> MGFLPQAQGGGAAASAKVSGTRFVIDGKTGYFAGTNSYWIGFLTNNRDVDTTLDHIASSGLKILRVWGFNDVNNQPSGNTVWFQRLASSGSQINTGPNGLQRLDYLVRSAETRGIKLIIALVNYWDDFGGMKAYVNAFGGTKESWYTNARAQEQYKRYIQAVVSR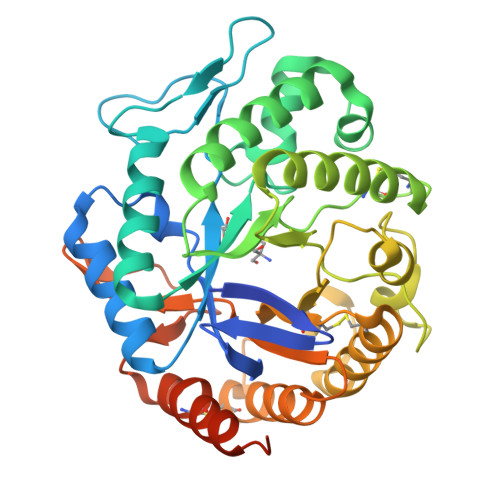YVNSPAIFAWELANEPRCKGCNTNVIFNWATQISDYIRSLDKDHLITLGDEGFGLPGQTTYPYQYGEGTDFVKNLQIKNLDFGTFHMYPGHWGVPTSFGPGWIKDHAAACRAAGKPCLLEEYGYESDRCNVQKGWQQASRELSRDGMSGDLFWQWGDQLSTGQTHNDGFTIYYGSSLATCLVTDHVRAINALPAGDEQKLISEEDLNSAVDHHHHHH>MGSDKIHHHHHHMVLTVTLNPALDREIFIEDFQVNRLYRINDLSKTQMSPGGKGINVSIALSKLGVPSVATGFVGGYMGKILVEELRKISKLITTNFVYVEGETRENIEIIDEKNKTITAINFPGPDVTDMDVNHFLRRYKMTLSKVDCVVISGSIPPGVNEGICNELVRLARERGVFVFVEQTPRLLERIYEGPEFPNVVKPDLRGNHASFLGVDLKTFDDYVKLAEKLAEKSQVSVVSYEVKNDIVATREGVWLIRSKEEIDTSHLLGAGDAYVAGMV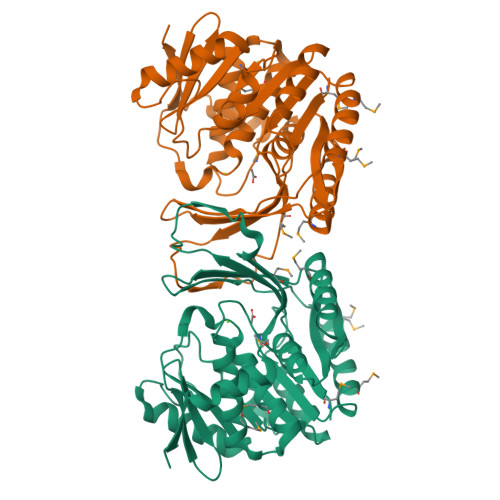YYFIKHGANFLEMAKFGFASALAATRRKEKYMPDLEAIKKEYDHFTVERVK[2x]>VQAVAVLKGDAGVSGVVKFEQASESEPTTVSYEIAGNSPNAERGFHIHEFGDATNGCVSAGPHFNPFKKTHGAPTDE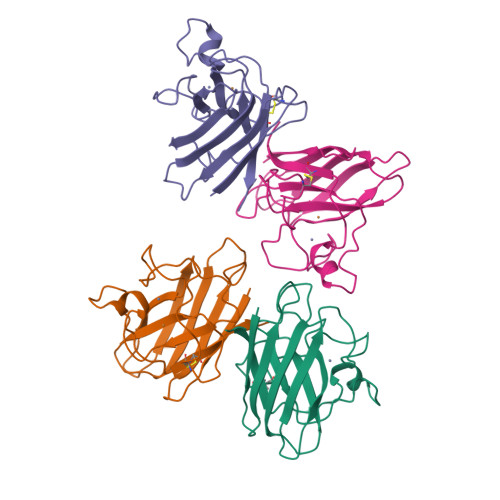VRHVGDMGNVKTDENGVAKGSFKDSLIKLIGPTSVVGRSVVIHAGQDDLGKGDTEESLKTGNAGPRPACGVIGLTN[4x]>SNPTTFSVEAIAAYTPVALIRLLNASGPLQPGHRVDIADARSIYTVGAAASAARARANHNANTIRRTAMFAETDPMTWLRPTVGLRRTFNPRII[6x];>[6x]PAGIIPTGNVLSTIEVCAHRCIFDFFKQIRSDDNSLYSAQFDILLGTYCNTLNFVRFLELGLSVACICTKFPELAYVRDGVIQFEVQQPMIARDGPHPVDQPVHNYMVKRIHKRSLSAAFAIASEALSLLSNTYVDGTEIDSSLRIRAIQQMARNLRTVLDSFERGTADQLLGVLLEKAPPLSLLSPINKFQPEGHLNRVARAALLSDLKRRVCADMFFMTRHAREPRLISAYLSDMVSCTQPSVMVSRITHTNTRGRQVDGVLVTTATLKRQLLQGILQIDDTAADVPVTYGEMVLQGTNLVTALVMGKAVRGMDDVARHLLDITDPNTLNIPSIPPQSNSDSTTAGLPVNARVPADLVIVGDKLVFLEALERRVYQ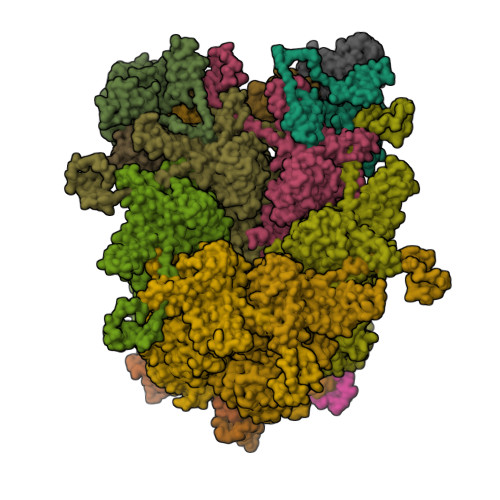ATRVAYPLIGNIDITFIMPMGVFQANSMDRYTRHAGDFSTVSEQDPRQFPPQGIFFYNKDGILTQLTLRDAMGTICHSSLLDVEATLVALRQQHLDRQCYFGVYVAEGTEDTLDVQMGRFMETWADMMPHHPHWVNEHLTILQFIAPSNPRLRFELNPAFDFFVAPGDVDLPGPQRPPEAMPTVNATLRIINGNIPVPLCPISFRDCRGTQLGLGRHTMTPATIKAVKDTFEDRAYPTIFYMLEAVIHGNERNFCALLRLLTQCIRGYWEQSHRVAFVNNFHMLMYITTYLGNGELPEVCINIYRDLLQHVRALRQTITDFTIQGEGHNGETSEALNNILTDDTFIAPILWDCDALIYRDEAARDRLPAIRVSGRNGYQALHFVDMAGHNFQRRDNVLIHGRPVRGDTGQAIPITPHHDREWGILSKIYYYIVIPAFSRGSCCTMGVRYDRLYPALQAVIVPEIPADEEAPTTPEDPRHPLHAHQLVPNSLNVYFHNAHLTVDGDALLTLQELMGDMAERTTAILVSSAPDAGAATATTRNMRIYDGALYHGLIMMAYQAYDETIATGTFFYPVPVNPLFACPEHLASLRGMTNARRVLAKMVPPIPPFLGANHHATIRQPVAYHVTHSKSDFNTLTYSLLGGYFKFTPISLTHQLRTGFHPGIAFTVVRQDRFATEQLLYAERASESYFVGQIQVHHHDAIGGVNFTLTQPRAHVDLGVGYTAVCATAALRCPLTDMGNTAQNLFFSRGGVPMLHDNVTESLRRITASGGRLNPTEPLPIFGGLRPATSAGIARGQASVCEFVAMPVSTDLQYFRTACNPRGRASGMLYMGDRDADIEAIMFDHTQSDVAYTDRATLNPWASQKHSYGDRLYNGTYNLTGASPIYSPCFKFFTPAEVNTNCNTLDRLLMEAKAVASQSSTDTEYQFKRPPGSTEMTQDPCGLFQEAYPPLCSSDAAMLRTAHAGETGADEVHLAQYLIRDASPLRGCLPL;>[2x]SIQVTPRSIVINRMNNIQINPTSIGNPNNGLHMTYNNAAAAAAAAAAAAAAAAAAAAAAAAAAAAAAAASIQVTPRSIVINRMNNIQINPTSIGNPQVTIRLPLNNFKSTTQLIQQVSLTDFFRPDIEHAGSTVLILRHPTDLPALARHRAPPGRQTERLAEAWGQLLEASRAYVTSLSFIAACRAEEYTDKQAAEANRTAIVSAYGCSRMGARLIRFSECLRAMVQCHVFPHRFISFFGSLLEYTIQDNLCNITAVAKGPQEAARTDKTSTRRVTANIPACVFWDVDKDLHLSADGLKHVFLVFVYTQRRQREGVRLHLALSQLNEQCFGRGIGFLLGARICMYAAYTLIGTIPSESVRYTRRMERFGGYNVPTIWLEGVVWGGTNTWNEC;>[2x]AMPFEIEVLLPGELSPAETSALQKCEGKIITFSTLRHRASLVDIALSSYYINGAPPDTLSLLEAYRMRFAAVITRVIPGKLLAHAIGVGTPTPGLFIQNTSPVDLCNGDYICLLPPVYGSADSIRLDSVGLEIVFPLTIPQTLMREIIAKVVARAVEDLNLMFSINEGCLLILALIPRLLALLIPRLLALVTREAAQLIHPEAPMLMLPIYETISSWISTSSRLGDTLGTRAILRVCVFDGPSTVHPGDRTAVIQV;>AMPFEIEVLLPGEISPAETSALQKCEGKIITFSTLRHRASLVDIALSSYYINGAPPDTLSLLEAYRMRFAAVITRVIPGKLLAHAIGVGTPTPGLFIQNTSPVDLCNGDYICLLPPVFGSADEIRLDSVGLEIVFPLTIPQTLMREIIAKVVARAVERTAADVICYNGRRYELETNLQHRDGSDAAIRTLVLNLMFSINEGTTLILTLITRLLRFPIYEAISSWISTSSRLGDTLGTRAILRVCVFDGPSTVHPGDRTAVIQV[2x]>MNLIKEDMRVKVHMEGNVNGHAFVIEGEGKGKPYEGTQTANLTVKEGAPLPFSYDILTTAVHYGNRVFTKYPEDIPDYFKQSFPEGYSWERTMTFEDKGICTIRSDISLEGDCFFQNVRFKGTNFPPNGPVMQKKTLKWEPSTEKLHVRDGLLVGNINMALLLEGGGHYLCDFKTTYKAKKV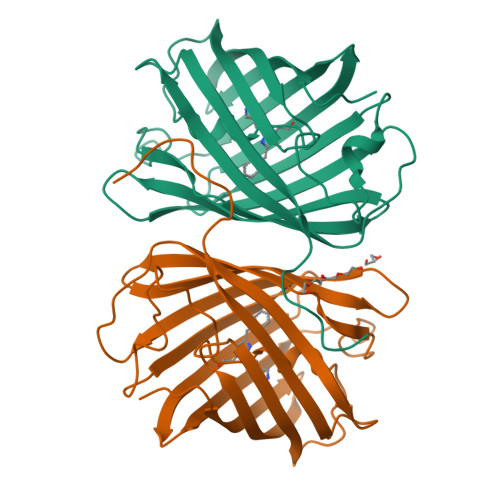VQLPDAHFVDHRIEILGNDSDYNKVKLYEHAVARYSPLPSQVWHHHHHH[8x]> MAPSRANTSVIVVGGGGTIGSSTALHLVRSGYTPSNVTVLDAYPIPSSQSAGNDLAKIMGVSLRNPVDLQLALEARQMWNEDELFKKFFHNTGRLDCAHGEKDIADLKSGYQALVDAGLDATNEWLDSEDEILKRMPLLSRDQIKGWKAIFSKDGGWLAAAKAINAVGEYLRDQGVRFGFYGAGSFKAPLLAEGVCIGVETVDGTRYYADKVVLAAGAWSPTLVELHEQCVSKAWVYGHIQLTPEEAARYKNSPVVYNGDVGFFFEPNEHGVIKVCDEFPGFTRFKMHQPFGAKAPKRISVPRSHAKHPTDTIPDASDVSIRRAIATFMPQFKNKKMFNQAMCWCTDTADAA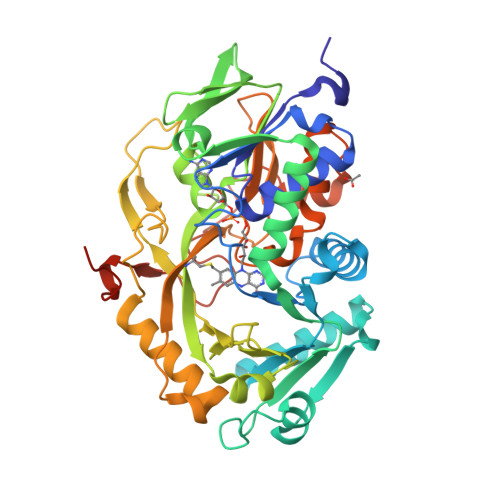LLICEHPEWKNFVLATGDSGHSFKLLPNIGKHVVELLEGTLADDLAHAWRWRPGSGDALKSRRSAPAKDLADMPGWNHDKPRANLLEHHHHHH>PLEAKFEEASLFKRIIDGFKDCVQLVNFQCKEDGIIAQAVDDSRVLLVSLEIGVEAFQEYRCDHPVTLGMDLTSLSKILRCGNNTDTLTLIADNTPDSIILLFEDTKKDRIAEYSLKLMDIDADFLKIEELQYDSTLSLPSSEFSKIVRDLSQLSDSINIMITKETIKFVADGDIGSGSVIIKPF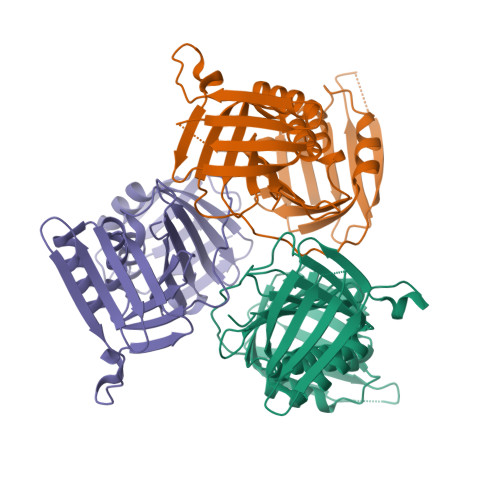VDMEHPETSIKLEMDQPVDLTFGAKYLLDIIKGSSLSDRVGIRLSSEAPALFQFDLKSGFLQFFLAPKFNDEE[3x]> SNALSPPAFRYQLTELARKAGKRIV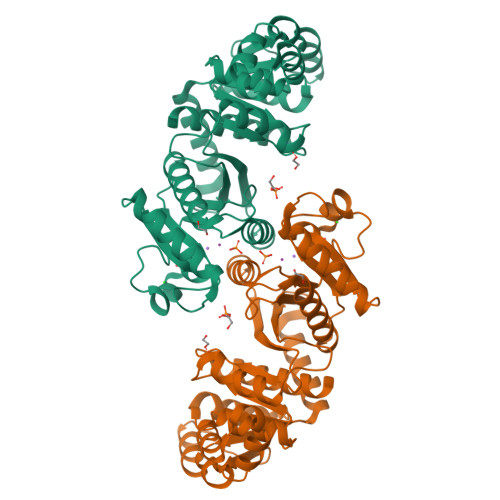LPEGDEPRTVKAAAICAERGIATCVLLGNPAEINRVAASQGVELGAGIEIVDPEVVRESYVGRLVELRKNKGMTETVAREQLEDNVVLGTLMLEQDEVDGLVSGAVHTTANTIRPPLQLIKTAPGSSLVSSVFFMLLPEQVYVYGDCAINPDPTAEQLAEIAIQSADSAAAFGIEPRVAMLSYSTGTSGAGSDVEKVREATRLAQEKRPDLMIDGPLQYDAAVMADVAKSKAPNSPVAGRATVFIFPDLNTGNTTYKAVQRSADLISIGPMLQGMRKPVNDLSRGALVDDIVYTIALTAIQSAQQQ> MNYI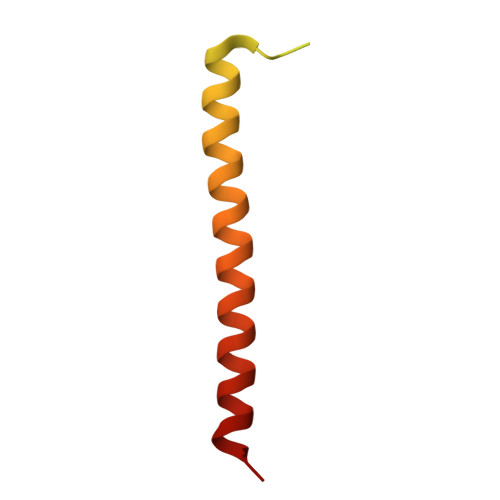YPVNQVDIIKASDFQSQEISSLEDVVSAKYSDIKMDTDIQVSQIMEMVSNPESLNPESLAKLQTTLSNYSIGVSLAGTLARKTVSAVETLLKS>[4x]MAKKDIMGDKTVRVRADLHHI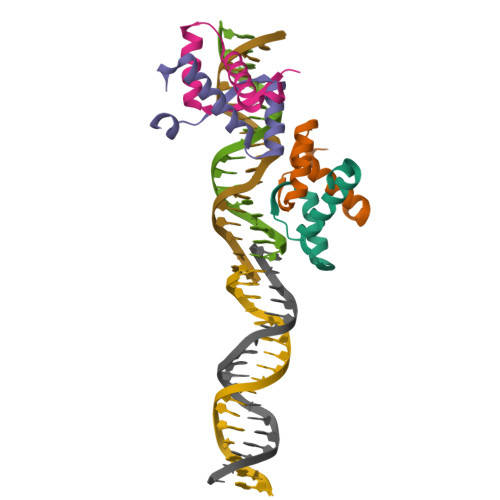IKIETAKNGGNVKEVMDQALEEYIRKYLPDKL>MSSAIKEVQGAPVKWVTNWTPEAIRGLVDQEKGLLDPRIYADQSLYELELERVFGRSWLLLGHESHVPETGDFLATYMGEDPVVMVRQKDKSIKVFLNQCRHRGMRICRSDAGNAKAFTCSYHGWAYDIAGKLVNVPFEKEAFCDKKEGDCGFDKAEWGPLQARVATYKGLVFANWDVQAPDLETYLGDARPYMDVMLDRTPAGTVAIGGMQKWVIPCNWKFAAEQFCSDMYHAGTTTHLSGILAGIPPEMDLSQAQIPTKGNQFRAAWGGHGSGWYVDEPGSLLAVMGPKVTQYWTEGPAAELAEQRLGHTGMPVRRMVGQHMTIFPTCSFLPAMNNIRIWHPRGPNEIEVWAFTLVDADAPAEIKEEYRRHNIRNFSAGGVFEQDDGENWVEIQKGLRGYKAKSQPLNAQMGLGRSQTGHPDFPGNVGYVYAEEAARGMYHHWMRMMSEPSWATLKP[6x];>MTNPSPHFFKTFEWPSKAAGLELQNEIEQFYYREAQLLDHRAYEAWFALLDKDIHYFMPLRTNRMIREGELEYSGDQDLAHFDETHETMYGRIRKVTSDVGWAENPPSRTRHLVSNVIVKE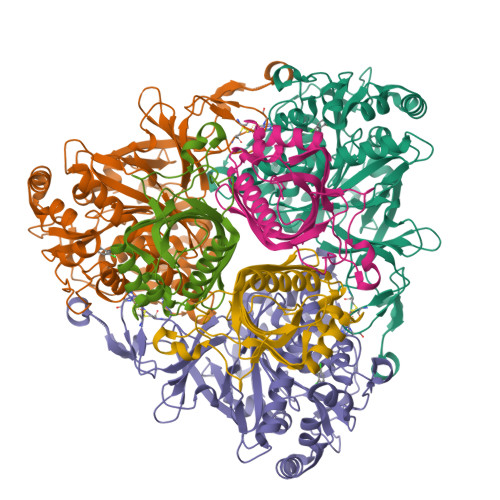TATPDTFEVNSAFILYRNRLERQVDIFAGERRDVLRRADNNLGFSIAKRTILLDASTLLSNNLSMFF[6x]> H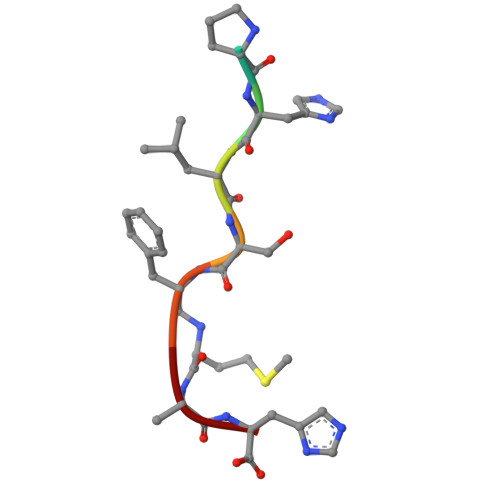PHLSXAH> MRLTQGCFSFLPDLTDQQIEKQVACAMSRGLAMNVEWTDDPHPRNNYWELWGLPLFDIKDPATVMFELNEARKSC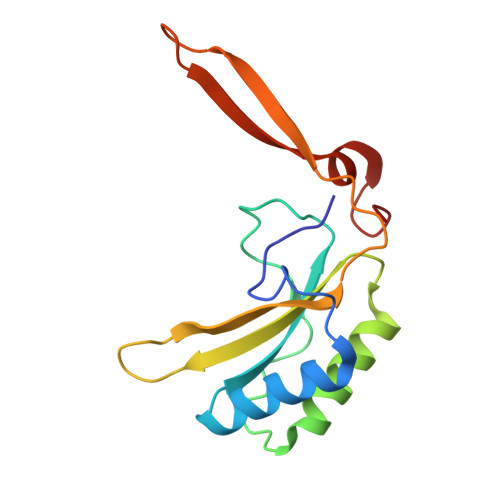AAGYIRMNAFDASYGTESCVMSFITNRPANEPGFYLDRTEGVGRQIVYSIKSYSVQANPEGSRY>SLFTSPFYKPIVQIPDANKKLKQSAGRGCTKMKFKVSKSNHDLLKSNKSYKLYLFSGFSIPFIYETVGHEAIDFPYPCELVFNGTKLEDNVKGLKKQNGTGNPANLTPYLKVPTEMNHLDLHYLNIDKEYSISC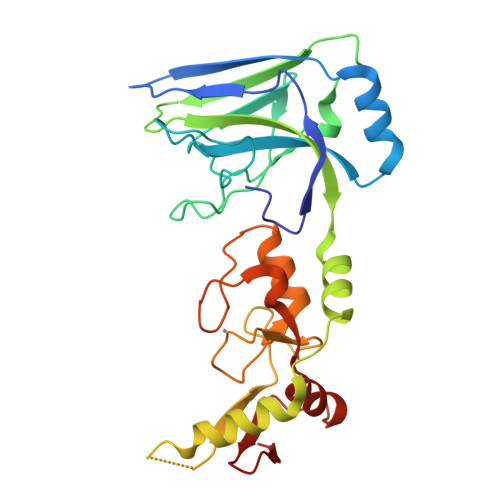FIVEVFSPEALLGKILKRPKIIKQATTAYIKRTLNEQDDDDIITTSTVLSLQCPISCTRMKYPAKTDQCKHIQCFDALWFLHSQSQVPTWQCPICQHPIKFDQLKISEFVDNIIQNCNEDVEQVEISVDGSWKPI[2x]> MTVNKLEPDNGTPNDELFTVAGMFDGSLYKLLLRMALPMFVGMLTQVTYAIADIFWLSHIDVTNSGIIAGVGLVFPVGMGLFAIANGIQIGMGSLLSRAIGMQRLDRAQRILSVGIIIALFFAIVITVLGYVYAQPLLRSLGATKSIIGYATEFYYYSLLTVFS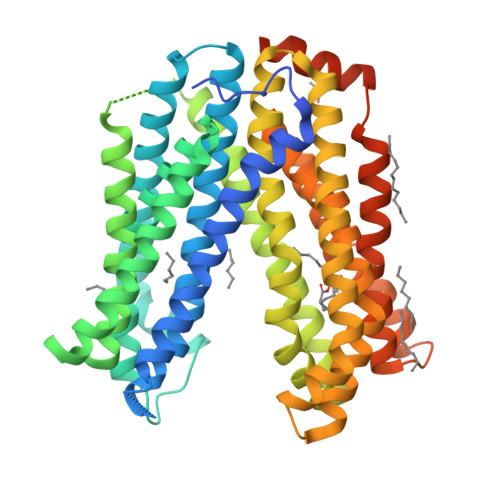IMLIGVMMGLFQGAGKIMVIMKASLLGALVNIMLDPIMIFVFDFGVKGVALASFLAQLSMVAYFIYTLMGLHIGLSIRIALRPFSWKIYREFLSVGMAQMLMQLIIAVGIVIYNFFIVRLDVNAMAAFTLTGRIDYFIITPMLAIATALLTVVGQNWGHGNVTRTLNAYWAAVALAFSIVLVLAVMHIVLAPWMYPLFTRVVAVSDYAVLQTRIMALALPFVAISLLASEYYQAIGKPWYSVLLTLMRHVFISVPVVYLLAIVLEMRITGVYFGAMSGTFVAALLAWRLLRLSPRLLRWNQEAVRSQHLDMEVAPADDDDKLAAAHHHHHHHHHH>[2x]MARPLEQAVAA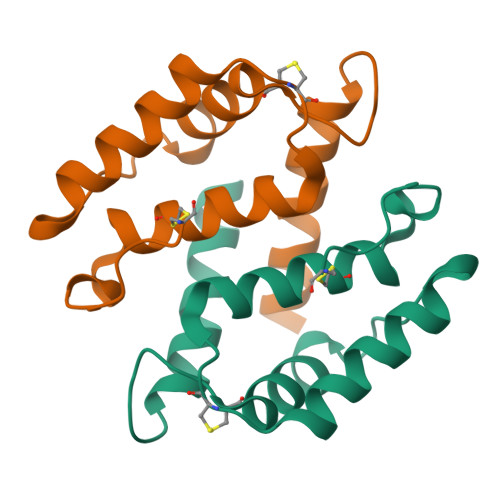IVCTFQEYAGRCGDKYKLCQAELKELLQKELATWTPTEFRECDYNKFMSVLDTNKDCEVDFVEYVRSLACLCLYCHEYFKDCPSEPPCSQ(2E)-3-(dimethylamino)-1-(2-hydroxyphenyl)prop-2-en-1-one 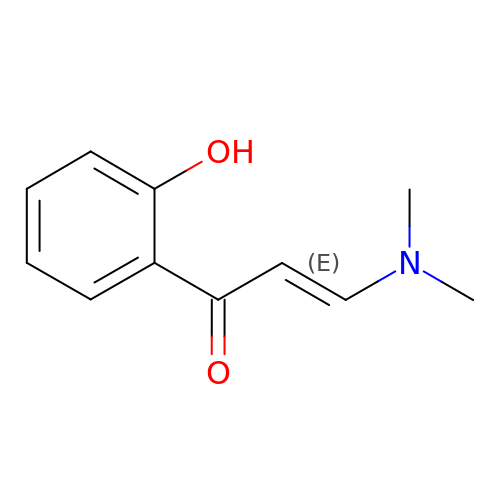| C11 H13 N O2 | SVBCOAAIOJDZNC-BQYQJAHWSA-N> SIKPGTYEVTSKVNGLHVGRPLAEDRSLLPKRIRVLPEDNNSGNSWVVEKDDDAYILYCKGAPVAPQEGKLFADLLGNMEDKKWIVTHQPQHGENVFTVVNASTEHGW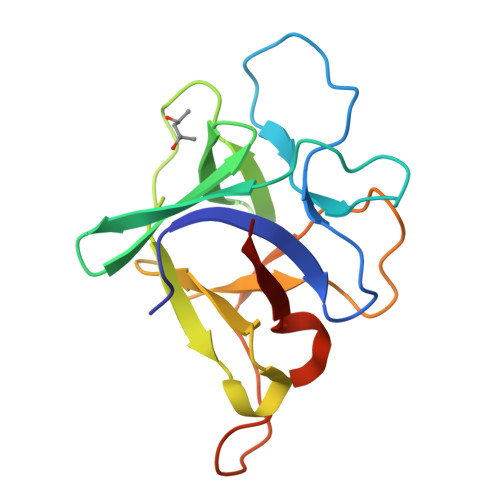VVPADAEELQQVEVRPLIAAPSYPPRYPATELFTFTQVESD> MTTAVARLQPSASGAKTRPVFPFSAIVGQEDMKLALLLTAVDPGIGGVLVFGDRGTGKSTAVRALAALLPEIEAVEGCPVSSPNVEMIPDWATVLSTNVIRKPTPVVDLPLGVSEDRVVGALDIERAISKGEKAFEPGLLARANRGYLYIDECNLLEDHIVDLLLDVAQSGENVVERDGLSIRHPARFVLVGSGNPEEGDLRPQLLDRFGLSVEVLSPRDVETRVEVIRRRDTYDADPKAFLEEWRPKDMDIRNQILEARERLPKVEAPNTALYDCAALCIALGSDGLRGELTLLRSARALAALEGATAVGRDHLKRVATMALSHRLRRDPLDEAGSTARVART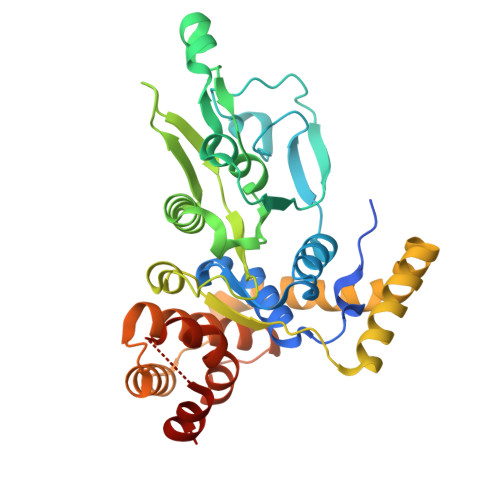VEETLP> MTLSTQRRALLAGFGKARGGQWTQEGIAALHSTTTTNAQVETQPDGELAESSADDASRLFQELSRRNRPNSAGTEPGPSPRPVLAQLPAAAELMERAAGTPSSQALYDLPTYLSVTHPHARVEPRNPAYDWRRSPQLEAGGPRRAALLLAVDAHMAAPESREALLRMAQLELAHLWYYQQHAAELPAAASPSASAASAASTATPDAAAAGQRRGGVAKQREAEPAAASTSAAAGDKAQAGAGTGTGAGAGAEAEAGDDDIFAAADRKARERAAAVEAATAAAASSAAKSLGRRGGRLPAELEARVRDMQLRYGMASRDAASVLRLLADSFSRRLPGGGRRLEGEAEAEAAVGLGEAEAEAGGDPTAALTWALSGGGRGGSGGTISGLSRHL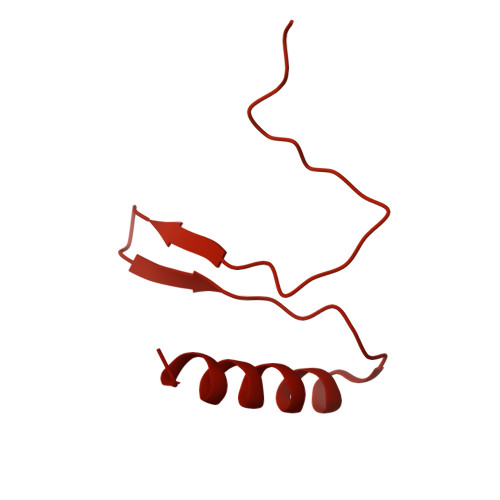AKQAAQAKAADRAIITAMQSLADAVNTASSSSSSATASSSTASSSGSSAYWAAHPALAYDQTLAARAHRQGLAWRAAAEAGPDGAASLSAAITALSASLRRPTSSPTSSASASSPPATPVLDLVLDYLQAKYADLLTAWETAARLREATERVSAAVARARATVPMSAVPPLPPALAAELERSWQNAAAAFRPALLQPLLQPAGSGAAARNSLAAAAASGSPALLQAQSSLTRPLDWAKAKALIEQHYAKQQQAAALAGATAAAEATAAAAAAASAAAAAGSPRGAVEALLQPLLQRAADRHRALLAGGDAAAAEAAAAAAAAAAHGSSTAAAGGAAPSEGAASVVCFRETLTLDASSAYANSSFDSRVTLEFNVDRLAAAEPGLGGAWGARFLERLLATPALPGSGRRIRGGGGSSGMFGRARASPAARAAANAAAYPVDVEHSFCRRTRTAALSTARYGSREANRKLLLEHYNELLRAAALAAAAGASAAV>ETTSCEFSVSPSGLAFCDKVVGYGPEAVKGQLIKAHYVGKLENGKVFDSSYNRGKPLTFRIGVGEVIKGWDQGILGSDGIPPMLTGGKRTLRIPPELAYGDRGAGCKGGSCLIPPASVLLFDIEYIGKA[5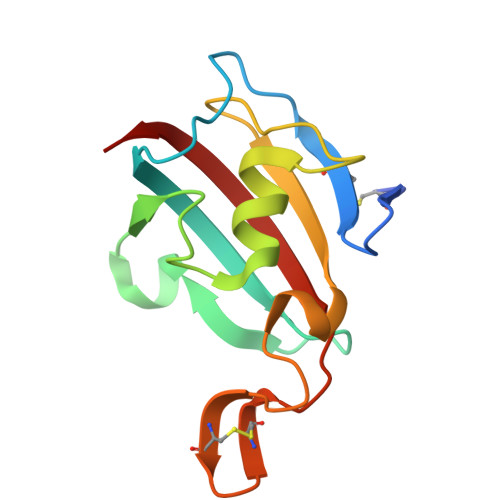x]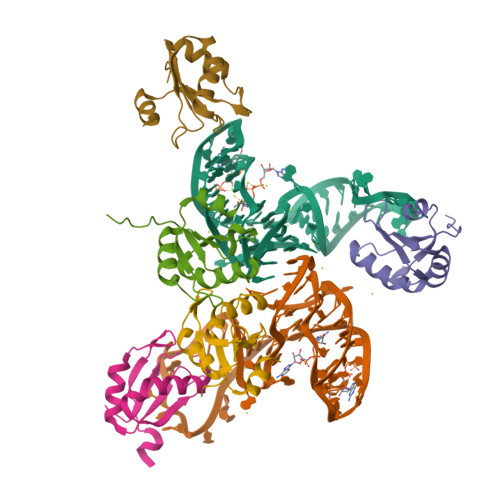>[5x]AVPETRPNHTIYINNLNEKIKKDELKKSLHAIFSRFGQILDILVSRSLKMRGQAFVIFKEVSSATNALRSMQGFPFYDKPMRIQYAKTDSDIIAKMK> MSQDPKIVNPQLWPNPNKLRFADLYKYQGVEMKKINDSIKNYKAAKFYIGGILGGCLVFKFFIDAAVDKYIFGENGNGGKFLEMQTINSNYDYYYNRQFQRMRYLTEDP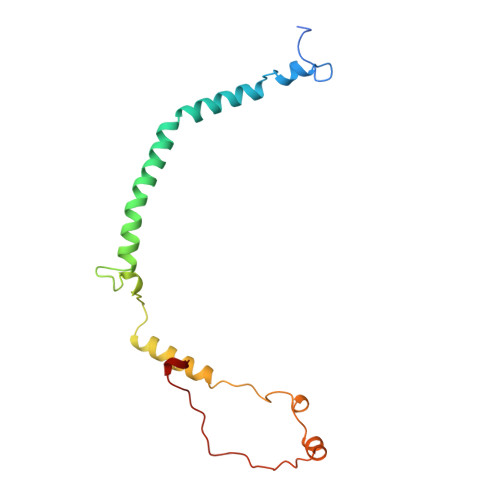AGDDPLQKTKDEHLVDLGFIPKVFGANVEVRKRAPHDKYL> GAPRELTWSQLIPAGAPPAPAPLPIHDLANALSEAGPAASQQSPNAPVVKALDGIEAKLPGYIVPLEISEAGLVTEFLLVPYYGACIHVPPPPSNQIVYVKTAKGVQMDELY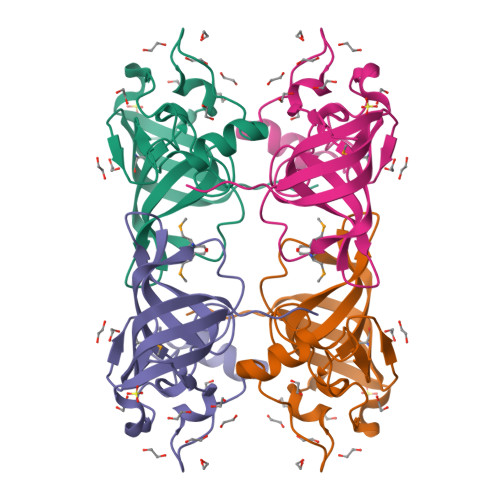QPFWVEGTFKVENASSELAAAGYRMQASKVTPYEYEGG>ARVAVLISGTGSNLQALIDSTREPNSSAQIDIVISNKAAVAGLDKAERAGIPTRVINHKLYKNRVEFDSAIDLVLEEFSIDIVCLAGFMRILSGPFVQKWNGKMLNIHPSLLPSFKGSNAHEQALETGVTVTGCTVHFVAEDVDAGQIILQEAVPVKRGDTVATLSERVKLAEHKIFPAALQLVASGTVQLGENGKICWVKEEHHHHHH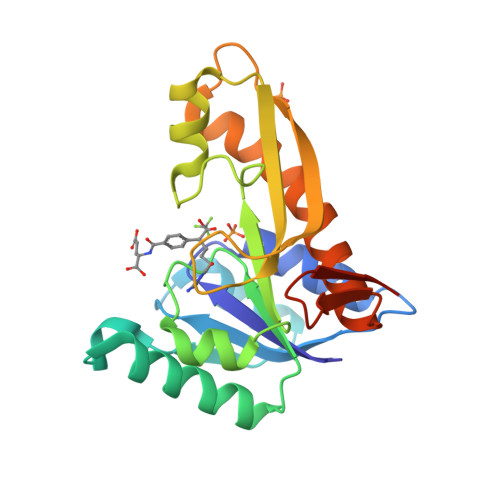[4x]>[2x]H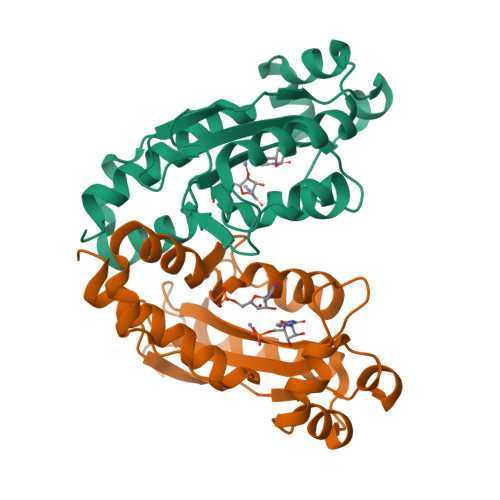MMAGNDSNLIWLDLEMTGLEPVEDVILEIAIIITDSELNILAQGPIFAISQTDDVLDNMNPWCIEHHGKSGLTQRCRDSEVSLAHATKESLAFVQEWVPQGKSPMCGNSIGQDRRFINKYMPDFEDHFHYRNLDVSTIKELAKRWKPEVLESVVKTGAHLALDDIKESIAELKVYRELFFKL>[2x]GPQDPYEINLMEELTLKGVTQYYAYVTERQKVHCLN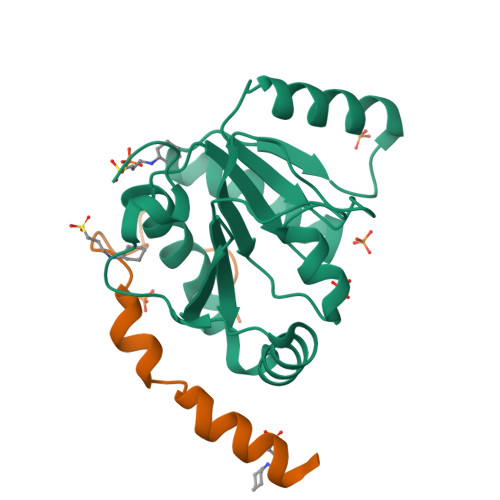TLFSRLQINQSIIFCNSSQRVELLAKKISQLGYSCFYIHAKMRQEHRNRVFHDFRNGLCRNLVCTDLFTRGIDIQAVNVVINFDFPKLAETYLHRIGRSGRFGHLGLAINLITYDDRFNLKSIEEQLGTEIKPIPSNIDKSLYVAEYHSEPVEDEKP;>[2x]GPHMADLFGDDIEEIPDTDFDFEGNLALFDKAAVFEEIDTYERR> ADSTITIRGYV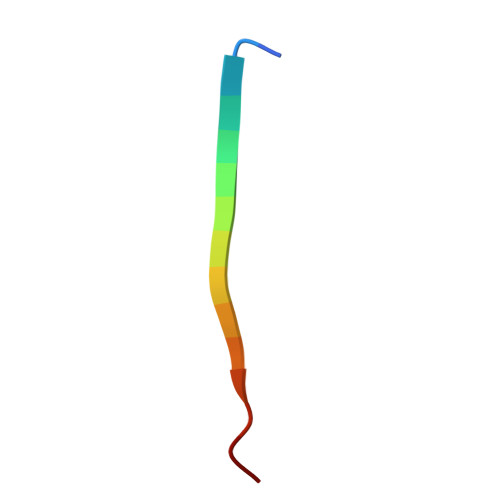RDNR> PKITLLTLIKTAEHWARQDIRTIEDSKLRALLTLCAVMTRKFSKSQLSLLCETHLRREGLGQDQAEPVLEVYQRLHSDKGGSFEAALWQQWDRQSLIMFITAFLNIALQL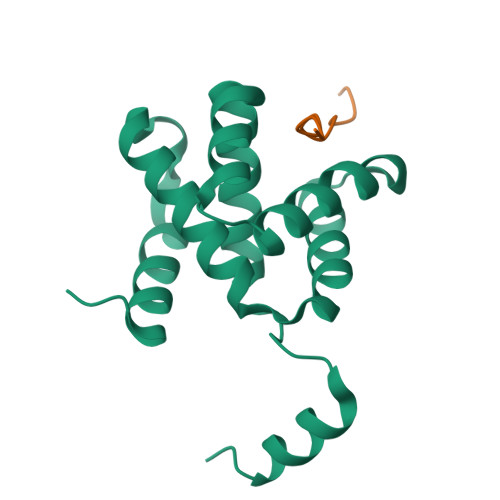PCESSAVVVSGLRTLVP;> PVFVPVPPPPLYPPP>TSDDHVPVDITDLLDRAAHDAARIYPDLDVSLVPSPTCIIVGLPAGLRLAVDNAIANAVKHGGATLVQLSAVSSRAGVEIAIDDNGSGVPEGERQVVFERFSRGSTASHSGSGLGLALVAQQAQLHGGTASL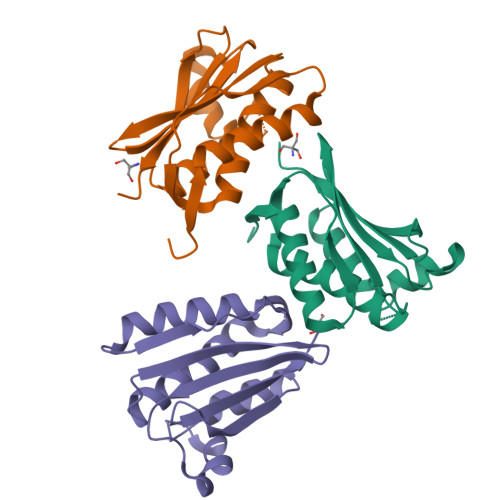ENSPLGGARLVLRLPGPS[3x]> SMSKTENAQKPHDRMAAYLESDMAAVSTLIRERMASKHAPRIPEVTAHLVEAGGKR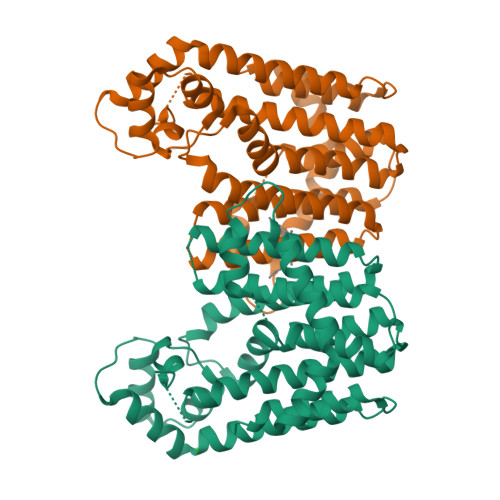LRPMLTLAAAHLCGYDGPFHINLAATVEFIHTATLLHDDVVDESGQRRGRPTANLLWDNKSSVLVGDYLFSRSFQLMVETGSLRVLDILANASATIAEGEVLQLTASQNLATTEEVYLQVVRGKTAALFSAATEVGGVIAGAPDDHVAALFEYGDALGIAFQIVDDLLDFQGDAGAIGKNIGDDFRERKLTMPLIKAVAKADAEERAFWVRTIEKGKQEEGDLQHAIALLHKHAALTDTSVVARTQAARAKAALAPLPAHPVKDMLVDLADYVVERIN>MSGSHHHHHHSGSMSERPSDLVVNRLVLFVVKGTATSTHATVKPLILLEELGVPHDIYVVEKVSAPWFSEINPHKMVPAILDRSPDGRDTLRAWESTSTLMYIADAYDKDGTFGGRNVQERSEINNWLTLHTAALGPTAKYWLYFYKLHPEKLPKTIEKLRSNITVQYDILERRLNEPGQQYLALKDRPTIADIATLPFAMKSTAELFGLEFEKWPKLQEWSVRMGEREAVKRAWQRVA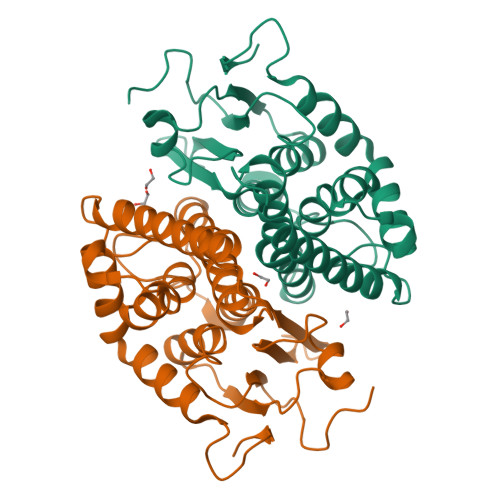GFGHGEKEYGMLEA[6x]(6-AMINOHEXYL)CARBAMIC ACID | C7 H16 N2 O2 | 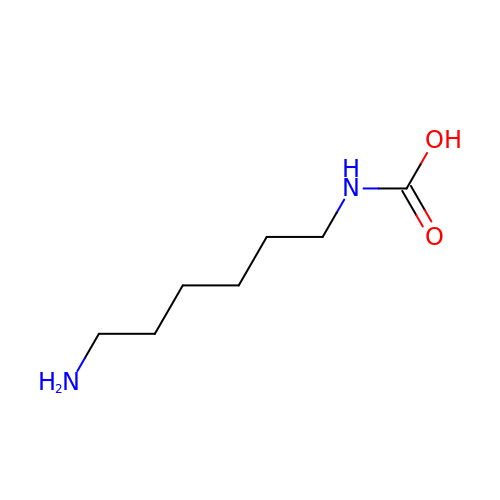HDIHOAXFFROQHR-UHFFFAOYSA-N>[8x]MKLQQLRYIVEVVNHNLNVSSTAEGLYTSQPGISKQVRMLEDELGIQIFARSGKHLTQVTPAGQEIIRI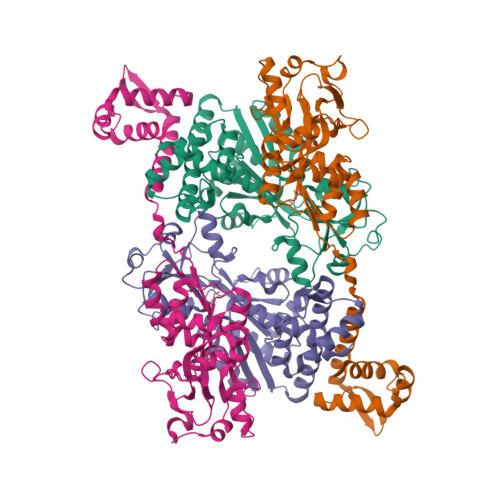AREVLSKVDAIKSVAGEHTWPDKGSLYVATTHTQARYALPGVIKGFIERYPRVSLHMHQGSPTQIAEAVSKGNADFAIATEALHLYDDLVMLPCYHWNRSIVVTPEHPLATKGSVSIEELAQYPLVTYTFGFTGRSELDTAFNRAGLTPRIVFTATDADVIKTYVRLGLGVGVIASMAVDPVSDPDLVKLDANGIFSHSTTKIGFRRSTFLRSYMYDFIQRFAPHLTRDVVDTAVALRSNEDIEAMFKDIKLPEK>[10x]SFPEVVELNVGGQVYFTRHSTLISIPHSLLWKMFSPK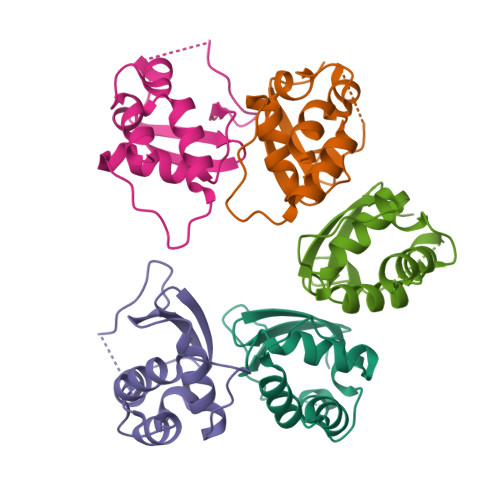RDTANDLAKDSKGRFFIDRDGFLFRYILDYLRDRQVVLPDHFPEKGRLKREAEYFQLPDLVKLLTPDEIKQSPDEF> MNNSSELIAVINGFRNSGRFCDISIVINDERINAHKLILSGASEYFSILFSNNFIDSNEYEVNLSHLDYQSVNDLIDYIYGIPLSLTNDNVKYILSTADFLQIGSAITECENYILKNLCSKNCIDFYIYADKYNNKKIESASFNTILQNILRLINDENFKYLTEESMIKILSDDMLNIKNEDFAPLILIKWLESTQQ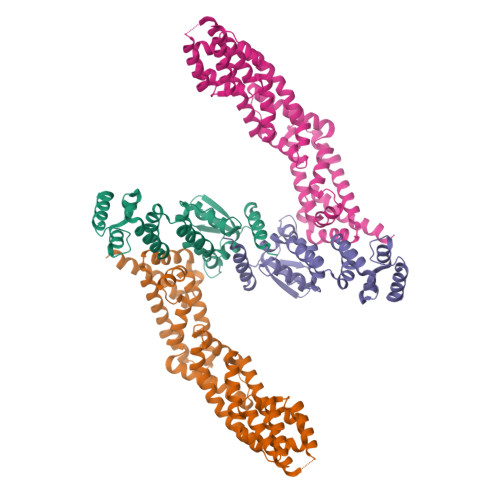SCTVELLRCLRISLLSPQVIKSLYSHQLVSSIYECITFLNNIAFLDESFPRYHGSKHHHHHH;> MTMDEKYVNSIWDLLKNAIQEIQRKNNSGLSFEELYRNAYTMVLHKHGEKLYTGLREVVTEHLINKVREDVLNSLNNNFLQTLNQAWNDHQTAMVMIRDILMYMDRVYVQQNNVENVYNLGLIIFRDQVVRYGCIRDHLRQTLLDMIARERKGEVVDRGAIRNACQMLMILGLEGRSVYEEDFEAPFLEMSAEFFQMESQKFLAENSASVYIKKVEARINEEIERVMHCLDKSTEEPIVKVVERELISKHMKTIVEMENSGLVHMLKNGKTEDLGCMYKLFSRVPNGLKTMCECMSSYLREQGKALVSEEGEGKNPVDYRQGLDDLKSRFDRFLLESFNNDRLFKQTIAGDFEYFLNLNSRSPEYLAENLYFQSHHHHHHDYKDDDDK>[2x]MASTDYHVDLTNCDREPIHIPGYIQPHGCLIACDNAMRMVLRHSENCGELLGLEGDLNGRTAEDVLGKRLVHDLRNALTVTGKTTRPAMLPAMETSDGRSFDISLHRYKSTTIIEFEPSDSDTQPLGTARKMVDRIREADSVESLISRTTRLVKATLGYDRVLIYRFEEDGAGKVVSEAKQPELESFLGQYFPA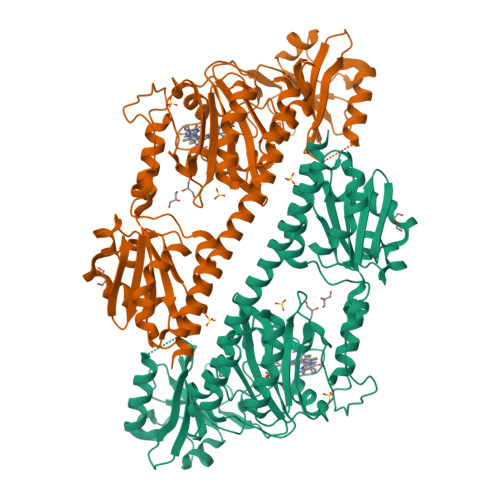SDIPQQARALYLKNTLRIISDASGTPIPVLPAVDVSGEPLDLSYAHLRNFSPIHCEYLRNMGVAASMSISVIVDDALWGLIVCHHCSPRVLSMPVRIAAAMFGEFFSMFLQVLKQKRRLDTINHAHAALDRFLRLAAHRANLEELLVDSFQDFARLIPCDGVGLWVGNNWHGHGATPPHDAIPRLARFVASVSEGRVWATHALSQAIPEAEIYADTAAGMLAIPISQVKSDYLLFFRKEIVQNLNWAGNPEKSYETGPMGDRLTPRKSFAIWKESVRLQAQPWSEADREIAETARIALVGVAFHHSELMAGLEYKHHHHHH> SRNTHYDFVITETKVTRLCHEKTILAVNGQFPGPTIYARKDDVVIVNVYNQGYKNITLHWHGVDQPRNPWSDGPEYITQCPIQPGANFTYKIIFTEEEGTLWWHAHSEFDRATVHGAIVIHPKRGTVYPYPKPHKEMPIILGEWWNADVEQILLESQRTGGDVNISDANTINGQPGDFAPCSKEDTFKMSVEHGKTYLLRVINAGLTNEMFFAVAGHRLTVVGTDGRYLRPFTVDYILISPGQTMNMLLEANCATDGSANSRYYMAARPFFTNTAVNVDDKNTTAIVEYTDAPPSASAGPP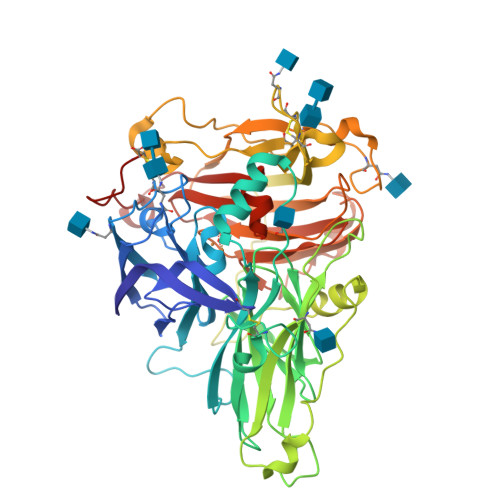DSPDLPAMDDIAAATAYTAQLRSLVTKEHPIDVPMEVDEHMLVTISVNTIPCEPNKTCAGPGNNRLAASLNNVSFMNPTIDILDAYYDSISGVYEPDFPNKPPFFFNFTAPNPPQDLWFTKRGTKVKVVEYGTILEVVFQDTAILGAESHPMHLHGFSFYVVGRGFGNFDKDKDPATYNLVDPPYQNTVSVPTGGWAAMRFRAANPGVWFMHCHFDRHTVWGMDTVFIVKNGKGPDAQMMPRPPNMPKC> GAMA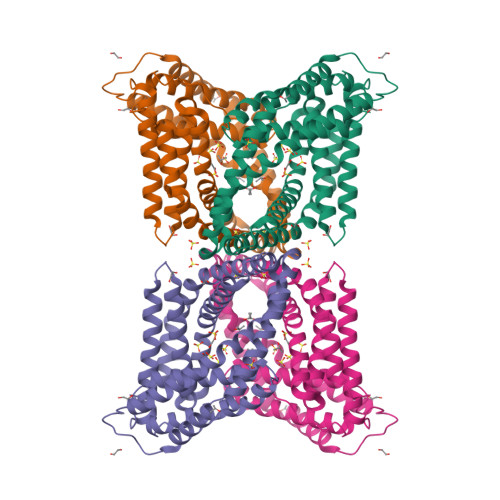SKLRLQLDAHASIHENVRRLLQFTTSIMEANEEGIRKDIDSEFLHDFRVAIRRSRSILRLLNGVFDPEKTAWMLAGLRELGKRTNDLRDSDVYLLRREEYTSLLPPSLRPALDPFFSDLEADKRLHHRQFCRYLTGREYSGFMTSLKEFIAEGELPDPETAPLAAEPTGDVAAKTIRKALKKVLVHGRRTGSETSDAELHELRIDCKKLRYLLEFFASLFPPKATAQVLRQMKTLQDNLGTFVDLTVQMEFLQSRLETIPADRGGISEAAAIGGLLTTLYRKREKVREHFHEIFSGFDSNETGELFDELLTGLA> KKSPSAGSGSNGGNKKISQEEGEDNGGEDNKKLRGALSSAILSEKPNVKWEDVAGLEGAKEALKEAVILPVKFPHLFKGNRKPTSGILLYGPPGTGKSYLAKAVATEANSTFFSVSSSDLVSKWMGESEKLVKQLFAMARENKPSIIFIDQVDALTGTRGEGESEASRRIKTELLVQMNGVGNDSQGVLVLGATNIPWQLDSAIRRRFERRIYIPLPDLAARTTMFEINVGDTPSVLTKEDYRTLGAMTEGYSGSDIAVVVKDALMQPIRKIQSATHFKDVSTEDDETRKLTPSSPGDDGAIEMSWTDIEADELKEPDLTIKDFLKAIKSTRPTVNEDDLLKQEQF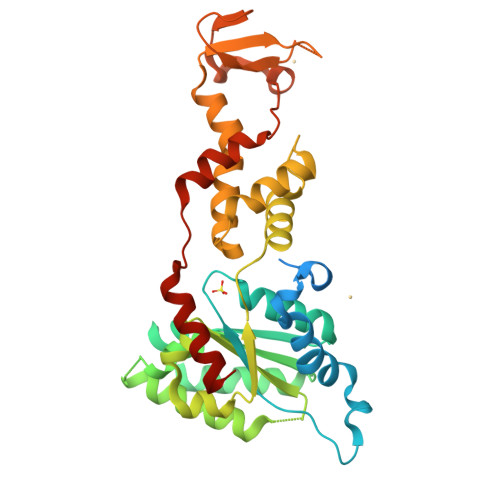TRDFGQEGN>[2x]MPGLFLTLEGLDGSGKTTQARRLAAFLEAQGRPVLLTREPGG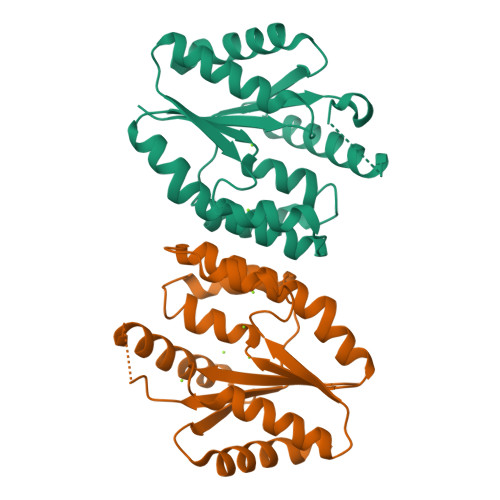GLPEVRSLLLTQELSPEAEYLLFSADRAEHVRKVILPGLAAGKVVISDRYLDSSLAFQGYGRGLPLPWLREVAREATRGLKPRLTFLLDLPPEAALRRVRRPDRLEGLGLEFFRRVREGYLALARAEPGRFVVLDATLPEEEIARAIQAHLRPLLP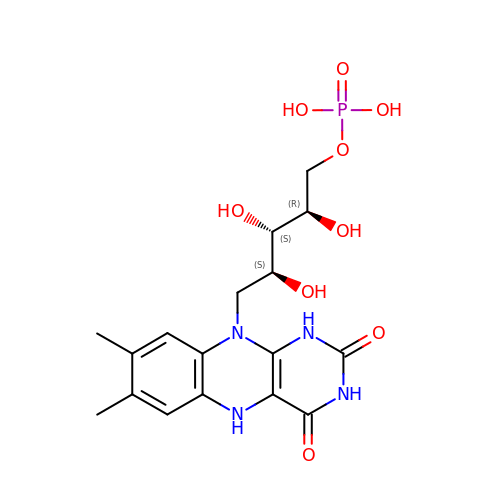1-DEOXY-1-(7,8-DIMETHYL-2,4-DIOXO-3,4-DIHYDRO-2H-BENZO[G]PTERIDIN-1-ID-10(5H)-YL)-5-O-PHOSPHONATO-D-RIBITOL | C17 H23 N4 O9 P | YTNIXZGTHTVJBW-SCRDCRAPSA-N> QRRLYDQAKAALAKGNSAPYMASRSALRDYPLEPYLAYDELTHRLKSASNEEVERFLTEHGDLPQIGWLKLRWLRLLADRGDWKTFVNYYDPKLNFTELDCLYGQYQLGHGQKAEGYATSERLWLVGKSQPAACDTLFGLWQGEGQLTEEKVWKRLKLAAEARNYSLASHLAQRLPTLGNQGALMVSVAQNPAQLSQTGRFSQ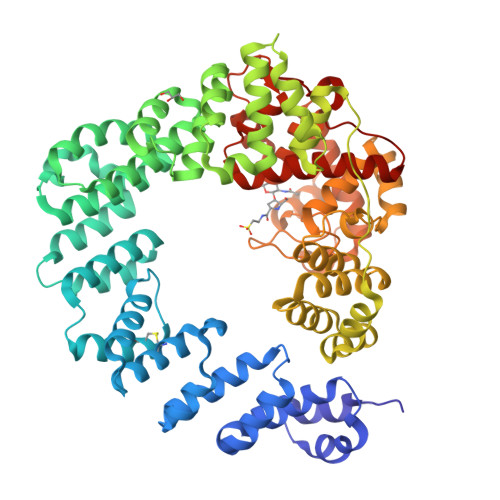RDHATADVVGLGLRRLARQDPEKALSLLDYYSSALPFSSDEKVAIAREIGLSLAKRFDPRALPLMTQYDPGLRDNTVTEWRTRLLLRLGRWDEAYALTRKLPQDLAATSRWRYWQARSLQLAQPNSKEPIALYQKLAGERDFYGFLAADRLSVPYKLGNRPAHIDPRVLQRVRNAASTRRAMEFFNRGEVINARREWYHAARLFDRDELIAQARLAYDMQWYFPAIRSISQAQYWDDLDIRFPMAHRATLVREAKNRGLHSSWIFAITRQQSAFMSDARSGVGATGLMQLMPGTAKETSRKFGIPLASTQQLIVPDVNIRLGAAYLSQVHSQFNGNRVLASAAYNAGPGRVRQWLKDTRHLAFDVWIETIPFDETRQYVQNVLSYAVIYGQKLNAPQPIVDWHERYFDDF> MAPVQLENHQLVPPGGGGGGSGGPPSAPAPPPPGAAVAAAAAAAASPGYRLSTLIEFLLHRAYSELMVLTDLLPRKSDVERKIEIVQFASRTRQLFVRLLALVKWANNAGKVEKCAMISSFLDQQAILFVDTADRLASLARDALVHARLPSFAIPYAIDVLTTGSYPRLPTCIRDKIIPPDPITKIEKQATLHQLNQILRHRLVTTDLPPQLANLTVANGRVKFRVEGEFEATLTVMGDDPDVPWRLLKLEILVEDKETGDGRALVHSMQISFIHQLVQSRLFADEKPLQDMYNCLHSFCLSLQLEVLHSQTLMLIRERWGDLVQVERYHAGKCLSLSVWNQQVLGRKTGTASVHKVTIKIDENDVSKPLQIFHDPPLPASDSKLVERAMKIDHLSIEKLLIDSVHARAHQKLQELKAILRGFNANENSSIETALPALVVPILEPCGNSECLHIFVDLHSGMFQLMLYGLDQATLDDMEKSVNDDMKRIIPWIQQLKFWLGQQRCKQSIKHLPTISSETLQLSNYSTHPIGNLSKNKLFIKLTRLPQYYIVVEMLEVPNKPTQLSYKYYFMSVNAADREDSPAMALLLQQFKENIQDLVFRTKTGKQTRTNAKRKLSDDPCPVESKKTKRAGEMCAFNKVLAHFVAMCDTNMPFVGLRLELSNLEIPHQGVQVEGDGFSHAIRLLKIPPCKGITEETQKALDRSLLDCTFRLQGRNNRTWVAELVFANCPLNGTSTREQGPSRHVYLTYENLLSEPVGGRKVVEMFLNDWNSIARLYECVLEFARSLPDIPAHLNIFSEVRVYNYRKLILCYGTTKGSSISIQWNSIHQKFHISLGTVGPNSGCSNCHNTILHQLQEMFNKTPNVVQLLQVLFDTQAPLNAINKLPTVPMLGLTQRTNTAYQCFSILPQSSTHIRLAFRNMYCIDIYCRSRGVVAIRDGAYSLFDNSKLVEGFYPAPGLKTFLNMFVDSNQDARRRSVNEDDNPPSPIGGDMMDSLISQLQPPPQQQPFPKQPGTSGAYPLTSPPTSYH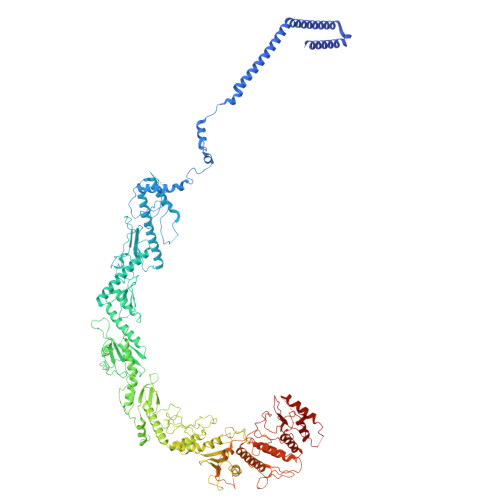STVNQSPSMMHTQSPGNLHAASSPSGALRAPSPASFVPTPPPSSHGISIGPGASFASPHGTLDPSSPYTMVSPSGRAGNWPGSPQVSGPSPAARMPGMSPANPSLHSPVPDASHSPRAGTSSQTMPTNMPPPRKLPQRSWAASIPTILTHSALNILLLPSPTPGLVPGLAGSYLCSPLERFLGSVIMRRHLQRIIQQETLQLINSNEPGVIMFKTDALKCRVALSPKTNQTLQLKVTPENAGQWKPDELQVLEKFFETRVAGPPFKANTLIAFTKLLGAPTHILRDCVHIMKLELFPDQATQLKWNVQFCLTIPPSAPPIAPPGTPAVVLKSKMLFFLQLTQKTSVPPQEPVSIIVPIIYDMASGTTQQADIPRQQNSSVAAPMMVSNILKRFAEMNPPRQGECTIFAAVRDLMANLTLPPGGRP>GPGSMCDEKKSSKNLKSVKIGYVNWGGETAATNVLKVVFEKMGYNAEIFSVTTSIMYQYLASGKIDGTVSSWVPTADKFYYEKLKTKFVDLG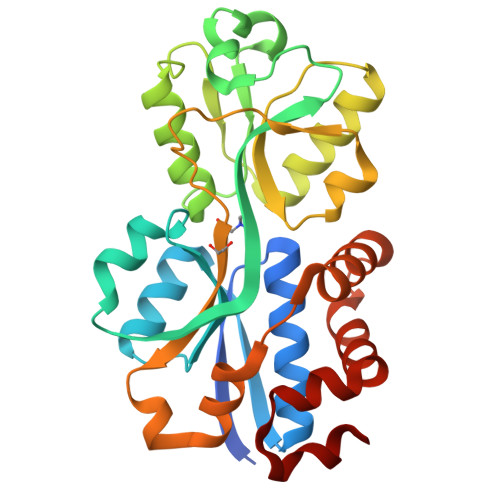ANYEGTIQGFVVPSYVPISSISELKGKGDKFKNKMIGIDAGAGTQIVTEQALNYYGLSKEYELVPSSESVMLASLDSSIKRNEWILVPLWKPHWAFSRYDIKFLDDPDLIMGGIESVHTLVRLGLENDDFDAYYVFDHFYWSDDLILPLMDKNDKEPGKEYRNAVEFVEKNKEIVKTWVPEKYKTLFD[4x]>[2x]GAMIVKRLLGWKKGEQNGQEEKWCEKAVKSLVKKLKKTGQLDELEKAITTQNVNTKCITIPRSLDGRLQVSHRKGLPHVIYCRLWRWPDLHSHHELRAMELCEFAFNMKKDEVCVNPYHYQRVETPVL

Smad proteins consist of an N-terminal MH1 domain, which binds to DNA, a linker region with phosphorylation sites for network regulatory inputs, and a C-terminal MH2 domain that is phosphorylated by the receptors and binds other Smad proteins, LDTFs, chromatin readers, and transcriptional co-activators and co-repressors. The receptors for TGF-β, nodal, activin, myostatin, and other family members are membrane serine/threonine kinases that phosphorylate and activate Smad2 and Smad3, whereas analogous receptors for the bone morphogenetic proteins (BMPs) preferentially phosphorylate and activate Smads 1, 5, and 8. These receptor-activated Smads (R-Smads) form heterotrimeric complexes with Smad4, which is required for the transcriptional regulation of most target genes. Focusing on the human and mouse Gsc promoter, here we identify specific Smad-binding GC-rich motifs and provide the X-ray crystal structures of Smad3 and Smad4 bound to several of these motifs. The structures determined here reveal that the β-hairpin is flexible and adaptable to bind with high-affinity several variants of the consensus sequence GGC(GC)|(CG), which we refer to as 5GC SBE.

The GC-rich region of Gsc contains a conserved GGCTG sequence, which resembles the GTCT-AGAC SBE. This GGCTG motif bound Smad3 and Smad4 MH1 domains with high affinity in the EMSA experiments. The Smad3 MH1 domain complex with the GGCT oligonucleotide was refined at 2.12 Å resolution (space group I41). Most of the hydrogen bonds with the GGCT site are very similar to those observed with Smad4. The main difference is that in the Smad3 complex no hydrogen bonds are observed from the ɛ-amino group of Lys81 to the G6 nucleotide. In this complex, we also detected several tightly bound water molecules at the protein–DNA interface that contribute to the stabilization of the interactions.> SLADAVTAWFPENKQSDVSQIWHAFEHEEHANTFSAFLDRLSDTVSARNTSGFREQVAAWLEKLSASAELRQQSFAVAADATESCEDRVALTWNNLRKTLLVHQASEGLFDNDTGALLSLGREMFRLEILEDIARDKVRTLHFVDEIEVYLAFQTMLAEKLQLSTAVKEMRFYGVSGVTANDLRTAEAMVRSREENEFTDWFSLWGPWHAVLKRTEADRWAQAEEQKYEMLENEYPQRVADRLKASGLSGDADAEREAGAQVMRETEQQIYRQLTDEVLALR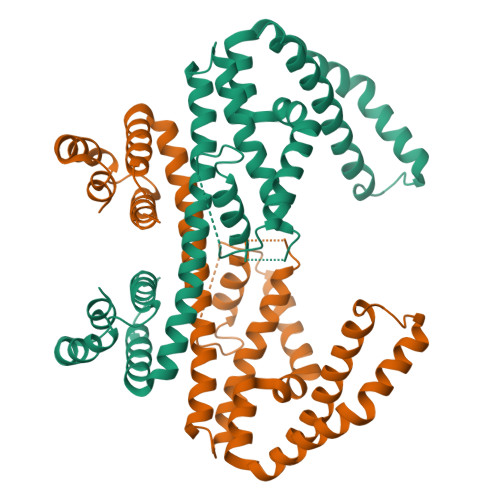LSENGSQLHHS>[2x]GKATTEEQKLIEDVNASFRAAMATTANVPPADKYKTFEAAFTVSYKRNLADAVSKAPQLVPKLDEVYNAAYNAADHAAPEDKYEAFVLHFSEALRIIAGTPEVHAVKPGA

We used the grass pollen allergen Phl p 6, which is a small globular protein of 11.8 kD that can be easily expressed in E. coli and is a known inducer of TH2 responses. We selected single point mutations that either stabilized or destabilized Phl p 6 without changing immunodominant T cell epitopes or the overall structure of the protein. Using these mutant proteins, we investigated the effect of fold-stability on antigen processing and presentation, as well as on immunogenicity and immune polarization in vitro and in vivo. Based on this concept, the overall fold-stability of an antigen has been suggested as an important protein intrinsic parameter that can influence immunogenicity and immune polarization.

In mutant S46Y, a buried polar amino acid was replaced by a hydrophobic amino acid. Such replacements have been referred to as “hydrophobic core packing” and reported to have stabilizing effects on the protein structure by increasing the overall hydrophobicity within the protein core. As predicted by MAESTRO, mutants E39L, N16M, and S46Y displayed an increased thermal stability compared to the WT protein (ΔT +8.8 to +14°C) whereas the destabilized mutant L89G was less heat stable (ΔT −5°C). A more detailed analysis with X-ray crystallography of mutant S46Y showed that the 3-dimensional structure was remarkably similar to that of the WT protein. The superimposition of the crystal structures of S46Y with Phl p 6 WT revealed that the overall fold is identical, with a total root-mean-square deviation of 0.42 A. As shown in Figure 5, the introduction of Tyr46 in the α2 helix, pointing into the central hydrophobic cavity, contributes to hydrophobic interactions with Phe42 within the α2 helix (and also Tyr68 in the neighboring α3 helix). In contrast, E39L and S46Y clearly showed delayed proteolytic processing, with S46Y being the most stable protein. We found that peptide 92–106 was much faster and more efficiently processed from L89G compared to the WT, whereas presentation was almost abrogated in the most rigid mutant S46Y. Despite the much slower protein degradation in vitro, S46Y turned out to be significantly more immunogenic in terms of IgG2a induction, while IgG1 levels, serum and cell bound IgE remained unaltered. On the contrary, the more stable mutant S46Y turned out to be more immunogenic and TH1 polarizing than the destabilized mutant L89G.5'-deoxy-5'-[4-({[(2,3-dihydroxy-5-nitrophenyl)carbonyl]amino}methyl)-1H-1,2,3-triazol-1-yl]adenosine | C20 H20 N10 O8 | 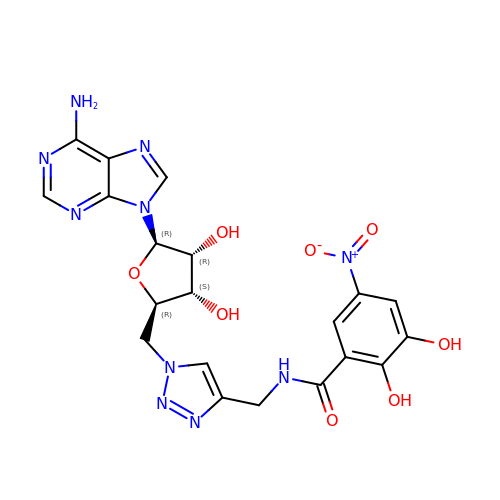KWTYQIOJSHGBKG-VXHCAWKWSA-N>[2x]SETRKTEVPSDKLELLLDIPLKVTVELGRTRMTLKRVLEMIHGSI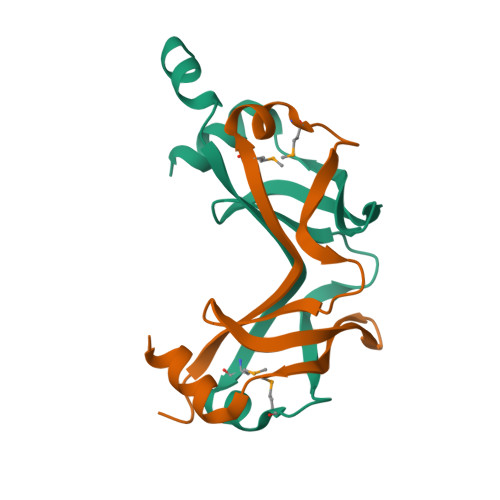IELDKLTGEPVDILVNGKLIARGEVVVIDENFGVRITEIVSPKERLELLNE>MDTPVMDSTDTDSTDIVIIGGGQAALSVAYYLRRSKYSFVMLDAEQTPGGAWLHGWDSLRLFSPSTWSSLSGWQMPPTGETYPSRDQVVDYLRHYESRYEFPVQRPVWVSAVNNLGDRLEVVSERQQWRARVVISATGTWRNPFIPAYPGADLFQGAQLHSAHYQSPAPFAGQKVLVVGGGNSGAQILAEVSRVADCTWVTTSEPIFLPDDVDGRVLFQRATDRWKAAQEGREIEQPVGGLGDVVMVPPVKEARERGALHAVRPFTRFTANGVVWADGTGSAVDAVIWCTGFRPALAHLQSLGVINPDGKVDLA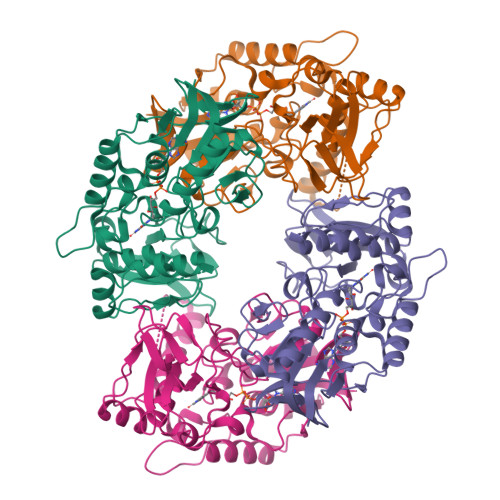GTRSLQEPRLWLLGYGEWTGLASATLIGVGRSARATAEEIIQYLDSA[2x]>MKHHHHHHQAKEKARYFTFLLYPESIPSDWELKLETLGVPMAISPLHDKDKSSIKGQKYKKAHYHVLYIAKNPVTADSVRKKIKLLLGEKSLAMVQVVLNVENMYLYLTHESKDAIAKKKHVYDKADI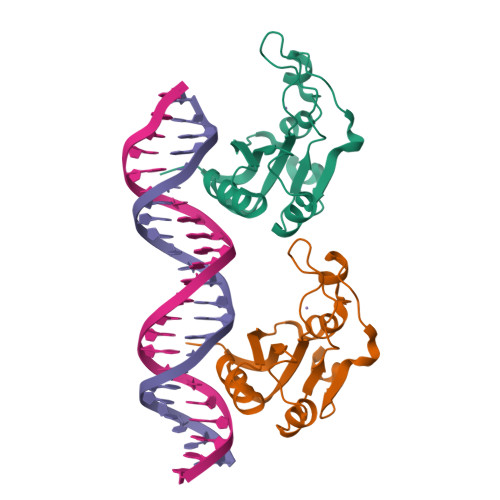KLINNFDIDRYV[4x]> MSTSHVDDEDVNSIAVAKTDGLNQLYNLVAQDYALTDTIECLSRMLHRGTIPLDTFVKQGRELARQQFLVRWH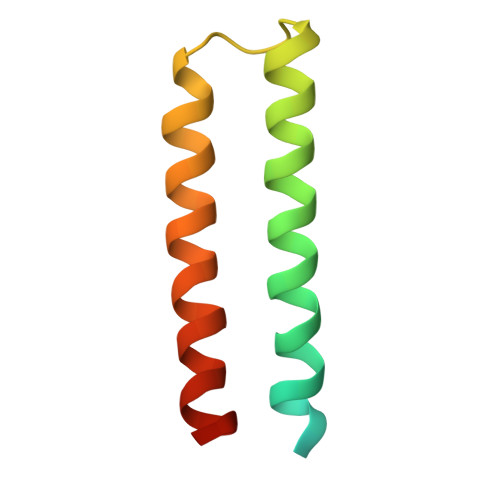IQRITSPLS> QTILPYPNGLYVINKGDGYMRTNDKDLIGTLLIESSTSGSIIQPRLRNTTRPLFNTSNPTIFSQEYTEARLNDAFNIQLFNTSTTLFKFVEEAPTN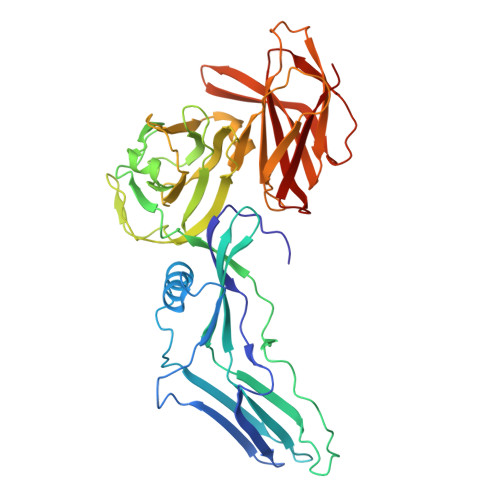KNISMKVYNTYEKYELINYQNGNIDDKAEYYLPSLGKCEVSDAPSPQAPVVETPVDQDGFIQTGPNENIIVGVINPSENIEEISTPIPDDYTYNIPTSIQNNACYVLFKVNTTGVYKITTKNNLPPLIIYEAIGSSNRNMNSNNLSNDNIKAIKYITGLNRSDAKSYLIVSLFKDKNYYIRIPQISSSTTSQLIFKRELGNISDLADSTVNILDNLNTSGTHYYTRQSPDVGNYISYQLTIPGDFNNIASSIFSFRTRNNQGIGTLYRLTESINGYNLITINNYSDLLNNVEPISLLNGATYIFRVKVTELNNYNIIFDAYRNS> RSDKELKFLVVDDGGTGRRIVRNLLKELGFNNVEEAEDGVDALNKLQAGGYGFVISDWNMPNMDGLELLKTIRADGAMSALPVLMVTAEAKKENIIAAAQAGASGYVVKPFT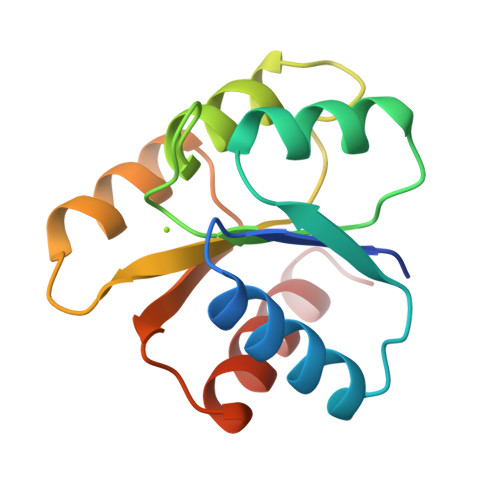AATLEEKLNKIFEKLGM>EFIRMYFEPGHYTVMENCGEFEVRVVRRGDISTYASVEYETQDGTASAGTDFVGRKGLLSFPPGVDEQRFRIEVIDDDVFEEDECFYIRLFNPSEGVKLAVP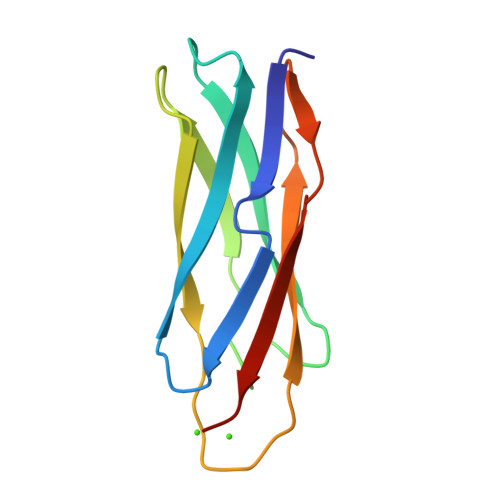MIATVMILDDDH[4x]>GNWLSTKALEQQTRDIPIEPKRGTIYDRNMKELAVSVTKYTVWCKPVEVEDKKEAAEKVAEILDEDYKDIYALISKKNMALVKVKRWIDDDKASQIRDAKLSGIWVAEDNQRYYPYGNFAPYVLGHTSSDATGISGVEMQYDKKLKGKPGKLIVSTDASGREIPQGMEKYYEPVQGNGLVLSIDEVIQHYTEKAVQKAYELNNAKKVTAIAMNPKTGDILALASKPDYDPNDSRTPIYPYYQEELEKYNDKDKIKGYYQMWRNPAVSDTYEPGSTFKLITSSSALEEGVIKDGEKFTCTGSVTVGGRKIKCWRHYRPHGTQEFKQAVQNSCNPVFVELGSRLGVGKMYDYIESFGLMDKTGIDLPGEAKGILYNEKNVGPVELATISFGQSISVTPIQLITAISSIANGGDLMQPRVVKSYTDNKGNITETVKPKKVRSVISKETSKKMLEIAESVVTEGGGKIAYIPGYRLGGKTGTAQKVIDGKYAPGKYICSFVGIAPCDDPQIVVLAIVDEPTGVSAFGSTTAGPIVKEIMNDSLKYLGVKPVY[2x]

Cephalosporins are members of the β-lactam family of antibiotics. These drugs achieve their bactericidal potency by irreversibly inhibiting penicillin-binding proteins (PBPs), particularly the transpeptidase (TPase) PBPs that cross-link cell wall peptidoglycan. Four annotated TPase PBPs exist in the genome of C. difficile R20291, a hypervirulent epidemic ribotype 027 strain: PBP1 (CDR20291_0712), PBP2 (CDR20291_0985), PBP3 (CDR20291_1067), and SpoVD (CDR20291_2544). A recent study found PBP1 and PBP2 are essential for vegetative growth in R20291, while SpoVD and PBP3 are essential for sporogenesis. Remarkably, in addition to C. difficile PBP2, we find this Zn2+-binding motif is also present in C. difficile PBP3 and SpoVD, meaning three of the four TPase PBPs, and all three class B PBPs in C. difficile have this motif.

Next, we determined the structures of PBP3 and SpoVD, at 2.40 Å and 2.20 Å resolution. Both SpoVD and PBP3 possess a canonical class B PBP fold that closely resembles Pseudomonas aeruginosa and E. coli PBP329,30. Like PBP2, the four residues in the Zn2+-binding motif of C. difficile PBP3 and SpoVD consist of an invariant His, a Cys from the X residue of the SXN motif, and two electron rich residues—in this case Cys instead of Asp. Importantly, we find Zn2+ binds in an almost identical manner as PBP2, suggesting Asp and Cys are interchangeable at the first and second position. The significance of the Asp → Cys substitution between SpoVD/PBP3 and PBP2 is unclear. Whereas the redox-sensitive cysteine in the SXN motif for PBP2 can potentially function as a sensor for environmental oxygen levels, the replacement of Asp for Cys in both sporulation specific PBPs (PBP3 and SpoVD) may further enhance the sensitivity and/or subject them to additional regulation. Nonetheless, SpoVD and PBP3 are very promising drug targets.Here, we have characterized an exceptionally large microvirus, Ebor, and provide crucial insights into long-standing mechanistic questions. Here, we report the structural analysis of the genome delivery process of a Microviridae phage, Ebor, along with its discovery and characterization. This phage, infecting a model aquatic Alphaproteobacterium Rhodobacter capsulatus, belongs to the microvirus taxon ‘Tainavirinae’ and recognizes the host via five Gokushovirinae-like trimeric protrusions. The capsid exhibits the triangulation number of T=1, being made of 60 copies of the major capsid protein. The core of the major capsid protein contains an 8-stranded antiparallel β-barrel (single jelly-roll fold), the fold shared among all Microviridae.

Subsequently, using a different purification method based on a sucrose gradient, we obtained a virus titre comparable to that obtained with CsCl gradient, as estimated by plaque assay. However, examination on the cryo-EM grid showed that all the particles had ejected the genome. The ejection likely occurred during the blotting procedure due to the reduced stability of the S120 variant. The icosahedrally averaged reconstruction of the empty particles led to a 3.3 Å resolution map, which notably lacked the trimeric protrusions. Otherwise, only subtle differences were observed between the major capsid protein models, built into the maps of native R120 and empty S120 particles. The respective models exhibited an average RMSDCα of 0.55 Å with the maximal RMSDCα of 2.3 Å occurring at the base of the protrusion. Here, the residues move towards the capsid interior as they are not repelled by the pressurized genome, thereby inducing the unfolding of the protrusion loop trimer.

> MSYQTKRNVRREARTLMGRFKAGKLAPVMAVPVKGSEGGMLSQSVSFELDPIAGRMATPITAEMCAVFVPVQACDALKNPEADYAGMTEIVREKLLSGNPLFVLEPETDVSKRCGVNPRSNNGLMRVNEIVRLAHNCAVNFLRRRRYVDAVQLTAANHSTTPAILSQTVLDRFNGALDPDPNVNGAVQLSMPDMRLPVASDAEKAVTAPLTVKRGNENRRLDAGISRLAAAEVAAATDAALYAVFGGREAGNVSLTDFYNAQKMDELTRVMRKICDDNPEYGEEMVLRWAHGLSVDPGRVPFLLAEKSVVLGRQIIGATDTAGVEDGVKRSDMAAQLSFTVPIPTTELGGIIVTFACIKPDETLSSQPHPILADHWRLDNFVADELALDPQPVMARELDYKVAQANETTVVFYTGLNELKKTYVSYGLCRALDPNTVESKNAVWQLEVPLSVTPETVLYPADLPQYPFADQQAEVCTYVVQSTAVMPTPMIFGPSPVEQLAVIETEDLFED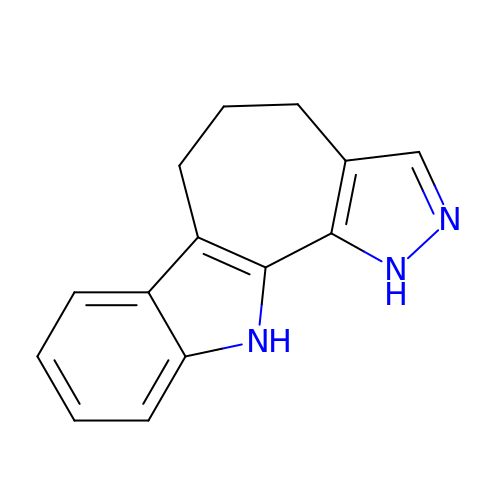4,5,6,11-tetrahydro-1H-pyrazolo[4',3':6,7]cyclohepta[1,2-b]indole | C14 H13 N3 | HBWXPQZQCDQNND-UHFFFAOYSA-N>[2x]MEAFEISDFKEHAKKKSMWAGALNKVTISGLMGVFTEDEDLMALPIHRDHCPALLKIFDELIVNATDHERACHSKTKKVTYIKISFDKGVFSCENDGPGIPIAKHEQASLIAKRDVYVPEVASCFFLAGTNINKAKDCIKGGTNGVGLKLAMVHSQWAILTTADGAQKYVQQINQRLDIIEPPTITPSREMFTRIELMPVYQELGYAEPLSETEQADLSAWIYLRACQCAAYVGKGTTIYYNDKPCRTGSVMALAKMYTLLSAPNSTIHTATIKADAKPYSLHPLQVAAVVSPKFKKFEHVSIINGVNCVKGEHVTFLKKTINEMVIKKFQQTIKDKNRKTTLRDSCSNIFVVIVGSIPGIEWTGQRKDELSIAENVFKTHYSIPSSFLTSMTRSIVDILLQSISKKDNHKQVDVDKYTRARNAGGKRAQDCMLLAAEGDSALSLLRTGLTLGKSNPSGPSFDFCGMISLGGVIMNACKKVTNITTDSGETIMVRNEQLTNNKVLQGIVQVLGLDFNCHYKTQEERAKLRYGCIVACVDQDLDGCGKILGLLLAYFHLFWPQLIIHGFVKRLLTPLIRVYEKGKTMPVEFYYEQEFDAWAKKQTSLVNHTVKYYKGLAAHDTHEVKSMFKHFDNMVYTFTLDDSAKELFHIYFGGESELRKRELCTGVVPLTETQTQSIHSVRRIPCSLHLQVDTKAYKLDAIERQIPNFLDGMTRARRKILAGGVKCFASNNRERKVFQFGGYVADHMFYHHGDMSLNTSIIKAAQYYPGSSHLYPVFIGIGSFGSRHLGGKDAGSPRYISVQLASEFIKTMFPAEDSWLLPYVFEDGQRAEPEYYVPVLPLAIMEYGANPSEGWKYTTWARQLEDILALVRAYVDKDNPKHELLHYAIKHKITILPLRPSNYNFKGHLKRFGQYYYSYGTYDISEQRNIITITELPLRVPTVAYIESIKKSSNRMTFIEEIIDYSSSETIEILVKLKPNSLNRIVEEFKETEEQDSIENFLRLRNCLHSHLNFVKPKGGIIEFNSYYEILYAWLPYRRELYQKRLMREHAVLKLRIIMETAIVRYINESAELNLSHYEDEKEASRILSEHGFPPLNHTLIISPEFASIEELNQKALQGCYTYILSLQARELLIAAKTRRVEKIKKMQARLDKVEQLLQESPFPGASVWLEEIDAVEKAIIKGRNTQWKFHHHHHH

However, for these theories to be broadly applicable, they need to be demonstrated for large and multimeric enzymes that catalyze complicated reactions. The enzyme used in this study is a type II DNA topoisomerase (Top2) from African swine fever virus (Asfv), a dimeric multi-subdomain enzyme (271 kDa) that catalyzes multistep reactions to modulate DNA topology. AsfvTop2 has been found to be involved in the early stage of viral gene replication, and also detected at the intermediate and late stages of infection. The domain composition of AsfvTop2 resembles that of the canonical Type IIA DNA topoisomerases (Top2), including the well-studied eukaryotic counterparts, which form homodimers. The catalytic process not only involves well-coordinated changes in protein quaternary structures to allow timely opening and closing of the N-, DNA-, and C-gates, but also ATP binding and sequential hydrolysis that relate the dimerization and catalytic activity of the ATPase domain to the mechanistic steps of the cycle.

We first performed the cryo-EM reconstruction of the full-length apo-AsfvTop2 without DNA or nucleotide. Furthermore, these primary conformational states are each sub-classified into two conformers, a and b, exhibiting local differences. The distribution of the three primary co-existing apo-conformers is approximately 1:4:2. Even though such differences are modest energetically, they do suggest that the closed state II is the most stable state, followed by the C-gate open state III and then the open state I. These thermodynamic properties are reflected in their structural properties described in the following sections. The changes in the Ia/IIa pair are mainly in the closing of the DNA-gate via the WHD subdomain. Conformers Ia/Ib were aligned globally with two apo-yeast Top2 structures. The results from the preceding section suggest that, even though the global conformation of apo-IIa is very similar to that of EDI-1, binding of DNA/inhibitor still induces small subdomain reorientations (Supplementary Movie 3: DNA-induced subdomain reorientation of AsfvTop2), yet coupled with substantial catalytically relevant conformational changes locally.>MSAQAAKVSKKELNSNHDGADETSEKEQQEAIEHIDEVQNEIDRLNEQASEEILKVEQKYNKLRQPFFQKRSE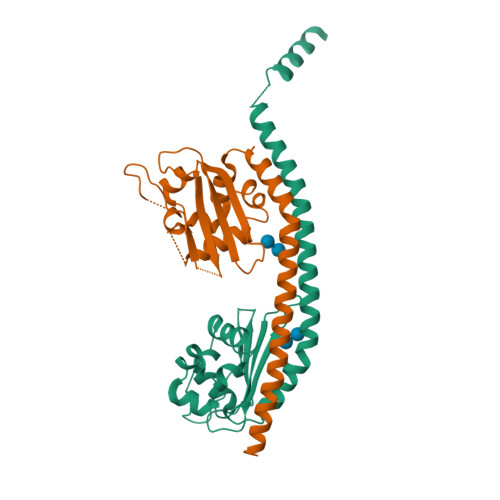LIAKIPNFWVTTFVNHPQVSALLGEEDEEAMHYLTRVEVTEFEDIKSGYRIDFYFDENPYFENKVLSKEFHMNESGDPSSKSTEIKWKSGKDMTKRSSQTQNKASRKRQHEEPESFFTWFTDHSDAGADELGEVIKDDIWPNPLQYYLVPDM[4x]>[8x]MKVVVQIKDFDKVPQALQSVLNLFLDLGNAEIEVVLHQSAIKALLLNSPTRSIIEELIKLNILI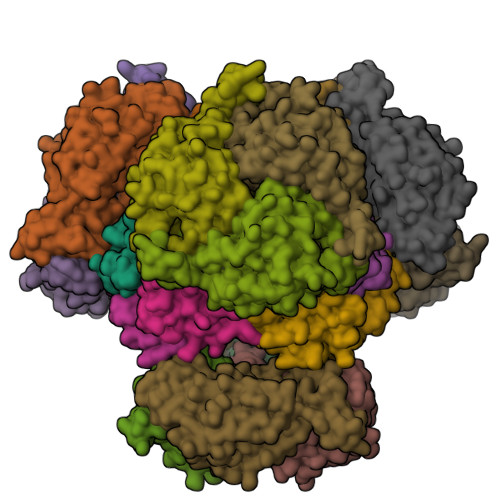VGCEHSIRSQNLDHRQLIDGIKIVRSGVGEIVRKQSEGWIYLAL;>MHHHHHHSGMSLRLERDGAVARLLIDRADRRNAFSLDMWQRLPELLAEASGDDALRVLVVKSANGGAFCAGADIAELLANKDDAAFHLANQQAINRAQYELARFRLPTVAMVEGDCIGGGCGIALACDMRIAAPAARFGITPAKLGLVYPLHDVKLLVDLVGPGQARRLMFTGGLIDANEAHRIGLVELLGESEDALVGQLATVSSFSTQAIKSFVRRVLDGQVADDTLSLCVFASATLGADFREGTGAFLEKRPPVF[8x]> ATCDDGRTTANAACCILFPILDDIQENLFDGAQCGEEVHESLRLTFHDAIGFSPTLGGGGADGSIIAFDTIETNFPANAGIDEIVSAQKPFVAKHNISAGDFIQFAGAVGVSNCPGGVRIPFFLGRPDAVAASPDHLVPEPFDSVDSILARMGDAGFSPVEVVWLLASHSIAAADKVDPSIPGTPFDSTPGVFDSQFFIETQLKGRLFPGTADNKGEAQSPLQGEIRLQSDHLL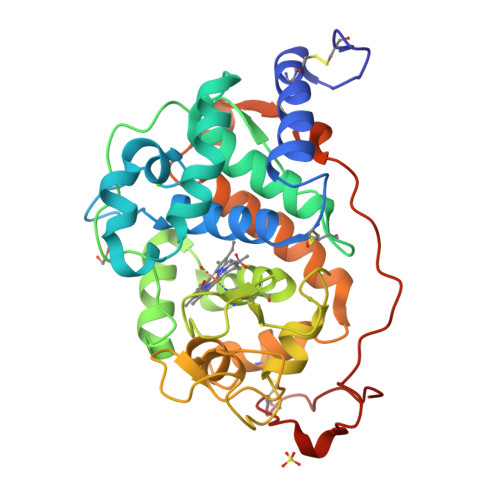ARDPQTACEWQSFVNNQPKIQNRFAATMSKMALLGQDKTKLIDCSDVIPTPPALVGAAHLPAGFSLSDVEQACAATPFPALTA[[(2~{R},3~{S},5~{R})-5-[4-[(4~{S})-4,5-bis(oxidanyl)pent-1-ynyl]-2-nitro-pyrrol-1-yl]-3-oxidanyl-oxolan-2-yl]methoxy-oxidanyl-phosphoryl] 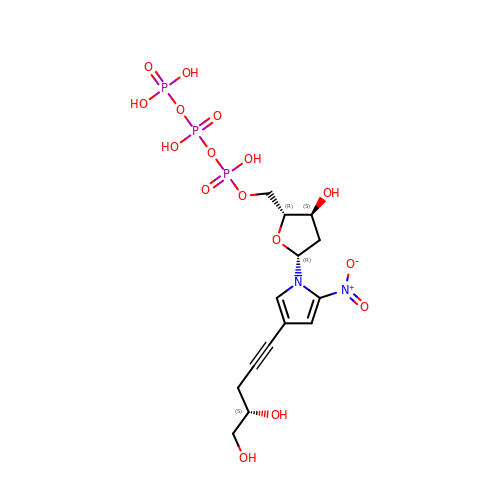phosphono hydrogen phosphate | C14 H21 N2 O16 P3 | JIVPAQSXWIKFCI-CIQGVGRVSA-N>GSMLELPPVASLKGKSITSAEQFSRADIYALIHLASAMQRKIDAGEVLNLLQGRIMTPLFFEDSSRTFSSFCAAMIRLGGSVVNFKVEASSINKGETLADTIRTLDSYSDVLVMRHPRQDAIEEALSVAQHPILNAGNGAGEHPTQALLDTLTIHSELGSVDGITIALIGDLKMGRTVHSLLKLLVRNFSIKCVFLVAPDALQMPQDVLEPLQHEIATKGVIIHRTHALTDEVMQKSDVLYTTRLQKERFMASTSDDAAALQSFAAKADITIDAARMRLAKEKMIVMHPLPRNDELSTTVDADPRAAYFRQMRY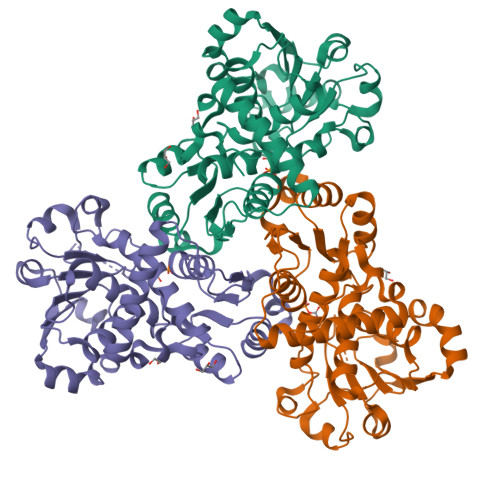GMFMRMAILWSVLA[6x]The RsiG–WhiG cognate pair is the only known example of a σ–anti-σ complex that is targeted by c-di-GMP. Here we show that the same σ–(c-di-GMP)–anti-σ switch has been co-opted during evolution to regulate distinct biological functions in unicellular and filamentous bacteria, controlling type IV pilus production in the genus Rubrobacter and the differentiation of reproductive hyphae into spores in Streptomyces. Moreover, we show that the anti-σ likely originated as a homodimer and evolved to become a monomer through an intragenic duplication event. Structural analyses revealed that these single-motif RsiGs form an antiparallel coiled-coil through homodimerization, enabling them to bind c-di-GMP in the same manner as the monomeric twin-motif RsiGs.

Two well-diffracting crystal forms of the RsiGRr protein were obtained. The structure of the second RsiGRr crystal form was solved by molecular replacement (MR) and refined to Rwork/Rfree values of 19.9%/26.8% to 2.55-Å resolution. The same antiparallel homodimer found in crystal form 1 was evident in this structure. The same RsiGRr crystal forms were obtained in the presence of c-di-GMP under identical crystallization conditions, but no nucleotide was visible in the structures. This appears to be due to the presence of Mg2+ ions, which were required for crystallization for both crystal forms. The Mg2+ ions in both apo structures are coordinated by D74, located at the C terminus of the E(X)3S(X)2R(X)3Q(X)3D motif. The tightly coordinated Mg2+ in the RsiGRr structure sterically disallows c-di-GMP binding. The presence of the same homodimers in both RsiGRr apo crystal structures, though they were obtained under very different conditions, supports that single-motif containing proteins can form the same antiparallel coiled-coil homodimer as observed in the monomeric twin-motif RsiGSv. Importantly, the finding also indicates that c-di-GMP binding is not necessary for dimerization of single-motif RsiG proteins. Interestingly, the regions that extend N and C terminal to the homodimeric RsiGRr central coiled-coils adopt short helical structures, which appear to depend on the crystal packing environment.

>GSHMARESAEEVWGGTEDLTSLSVEELKGLMARFDEEEKRISYRRRVMQGRIDVIRAEIVRRGGAVLSPEELARVLMGDVGDESE[3x]>[2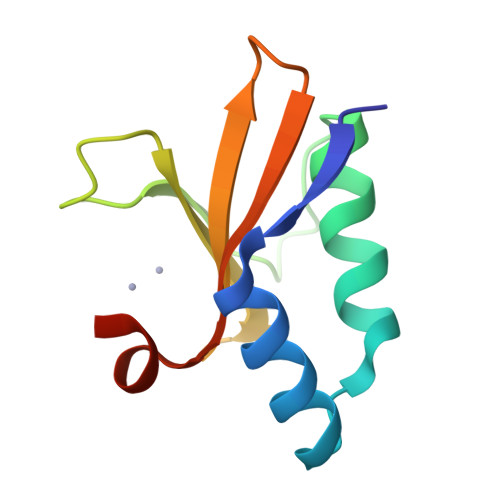x]MLTIETSKKFDKDLKILVKNGFDLKLLYKVVGNLATEQPLAPKYKDHPLKGGLKDFRECHLKPDLLLVYQIKKQENTLFLVRLGSHSELFLVPR2'-[(6R,6aR,11bR)-2-carbamimidoyl-6,6a,7,11b-tetrahydro-5H-indeno[2,1-c]quinolin-6-yl]-5'-hydroxy-4'-methoxybiphenyl-4-carboxylic acid | C31 H27 N3 O4 | 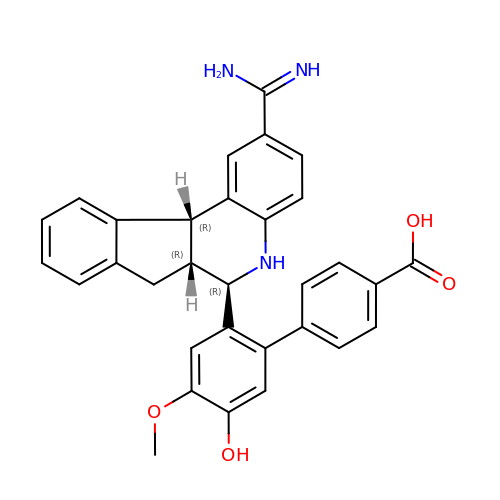UZOHOGNUODEPEP-USOMCTOXSA-N>[8x]MRGSHHHHHHGMTIFEKKPDFTLFLQTLSWEIDDQVGIEVRNELLREVGRGMGTRIMPPPCQTVDKLQIELNALLALIGWGTVTLELLSEDQSLRIV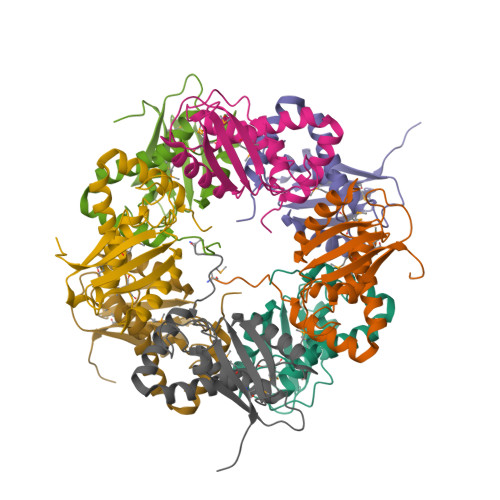HENLPQVGSAGEPSGTWLAPVLEGLYGRWVTSQAGAFGDYVVTRDVDAEDLNAVPRQTIIMYMRVRSSAT>[2x]MDERDALRISREIAGEVRKAIASMPLRERVKDVGMGKDGTPTKAADRVAEDAALEILRKERVTVVTEESGVLGEGDVFVALDPLDGTFNATRGIPVYSVSLCFSYSDKLKDAFFGYVYNLATGDEYYADSSGAYRNGERIEVSDAEELYCNAIIYYPDRKFPFKRMRIFGSAATELCFFADGSFDCFLDIRPGKMLRIYDAAAGVFIAEKAGGKVTELDGESLGNKKFDM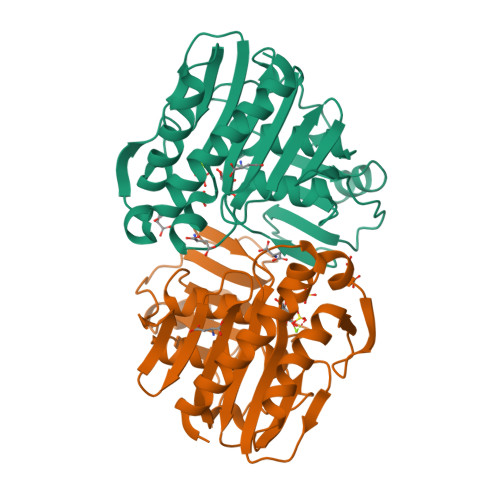QERLNIVAANEKLHPKLLELIK>[12x]GSLQTEKFDFGTMVQWAYDHKYAEESKIAYEYALAAGSDSNARAFLATNSQAKHVKDCATMVRHY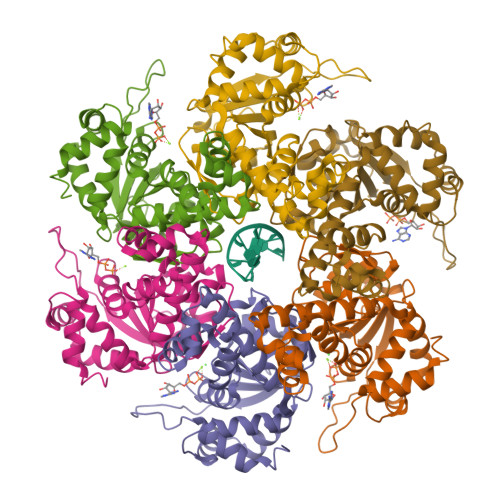LRAETQALSMPAYIKARCKLATGEGSWKSILTFFNYQNIELITFINALKLWLKGIPKKNCLAFIGPPNTGKSMLCNSLIHFLGGSVLSFANHKSHFWLASLADTRAALVDDATHACWRYFDTYLRNALDGYPVSIDRKHKAAVQIKAPPLLVTSNIDVQAEDRYLYLHSRVQTFRFEQPCTDESGEQPFNITDADWKSFFVRLWGRLDL> GPLGSLCGRVFKVGEPTYSCRDCAVDPTCVLCMECFLGSIHRDHRYRMTTSG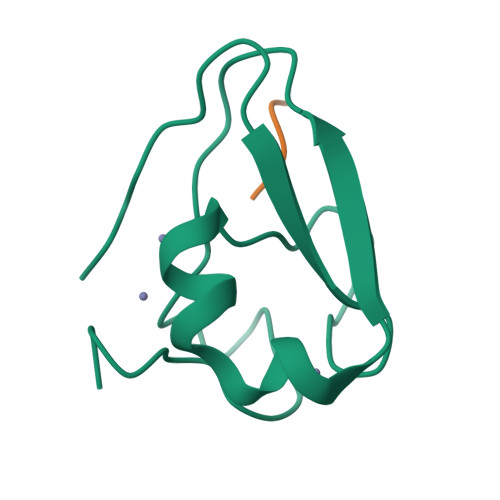GGGFCDCGDTEAWKEGPYCQKHE;> RIFS>[3x]MGASANALGMIETKGLVGAIEAADAMVKAANVQLVGKEQVGGGLV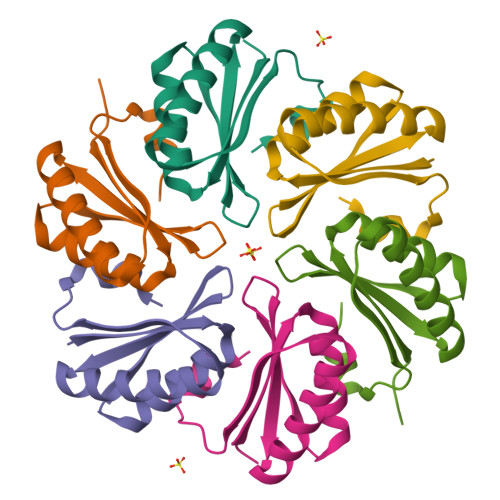TVMVRGDVGAVKAATDAGAAAAERVGELISVHVIPRPHFEVDAILPKVSAELEHHHHHH(3S)-3-methyl-1-(6-methylpyridin-2-yl)piperazine 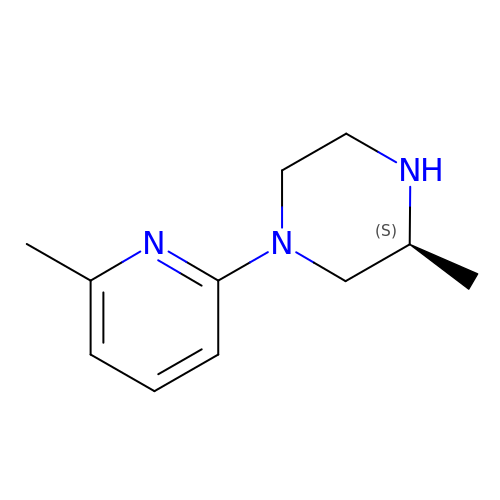| C11 H17 N3 | YCMYTWGABUXSEI-JTQLQIEISA-N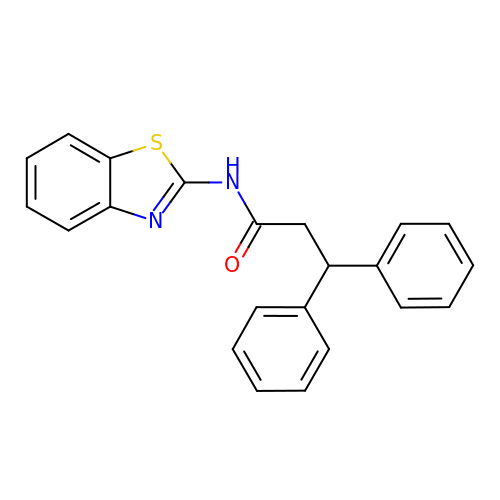~{N}-(1,3-benzothiazol-2-yl)-3,3-diphenyl-propanamide | C22 H18 N2 O S | GYQWKTIZRYVFEM-UHFFFAOYSA-N> QEGLDFPEYDGVDRVINVNAKNYKNVFKKYEVLALLYHEPPEDDKASQRQFEMEELILELAAQVLEDKGVGFG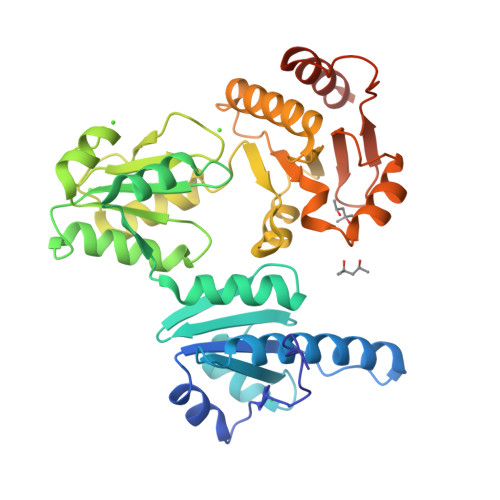LVDSEKDAAVAKKLGLTEVDSMYVFKGDEVIEYDGEFSADTIVEFLLDVLEDPVELIEGERELQAFENIEDEIKLIGYFKSKDSEHYKAFEDAAEEFHPYIPFFATFDSKVAKKLTLKLNEIDFYEAFMEEPVTIPDKPNSEEEIVNFVEEHRRSTLRKLKPESMYETWEDDMDGIHIVAFAEEADPDGFEFLETLKAVAQDNTENPDLSIIWIDPDDFPLLVPYWEKTFDIDLSAPQIGVVNVTDADSVWMEMDDEEDLPSAEELEDWLEDVLEGEINTEDDDDDDDD> AQELQTANEFTV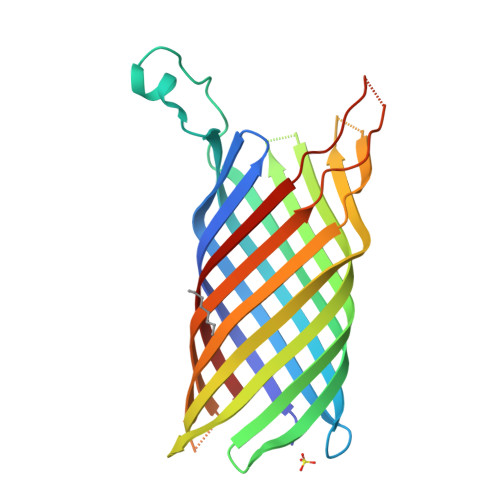HTDLSSISSTRAFLKEKHKAAKHIGVRADIPFDANQGIRLEAGFGRSKKNIINLETDENKLGKTKNVKLPTGVPENRIDLYTGYTYTQTLSDSLNFRVGAGLGFESSKDSIKTTKHTLHSSRQSWLAKVHADLLSQLGNGWYINPWSEVKFDLNSRYKLNTGVTNLKKDINQKTNGWGFGLGANIGKKLGESASIEAGPFYKQRTYKESGEFSVTTKSGDVSLTIPKTSIREYGLRVGIKF> GHITDEAKVPAYTLPAVLALKSGQPVTDAKSWTTKRRPEILAIYEAEVYGKSPARPPKLNYEVKSVEKQALGGKATRKIVTIFFSDKPDAPKMD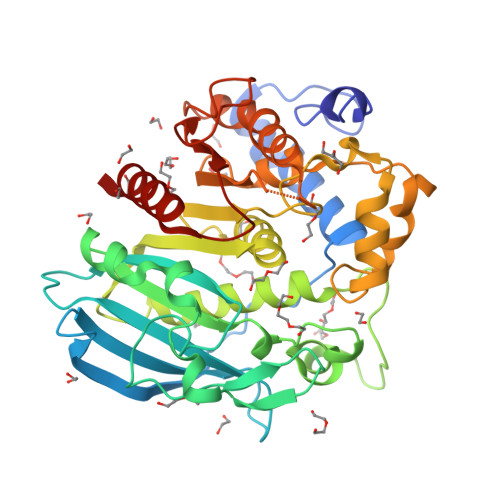LLLYLPAAAAKPAPVILGLSFGGIHTVANDPGVPLAEQWTRDNRKQPSAEKSRGGEASRWQVEKILAAGYGLATVYYEQIEPDFAGGMKYGIRPLFFKPGQTEPEPGDWGAVAAWAWGASRAMDYLEKDKDVDARRVGLIGHSRLGKAAIWAGAQDARFTFIISNESGEGGAAISRRDYGERTTALNTRFPHWFDGNYKKYNDRENEMPFDSHMALALMAPRGLYVASAEGDQWSDPKGEFLGAANASPVWELFGKKGIGTMTMPDLHEPVGDSVRYHIRAGKHDVTEYDWEQYLKFAKAQWG>MSGAMAALTAEHFAALQSLLKASSKDVVRQLCQESFSSSALGLKKLLDVTCSSLSVTQEEAEELL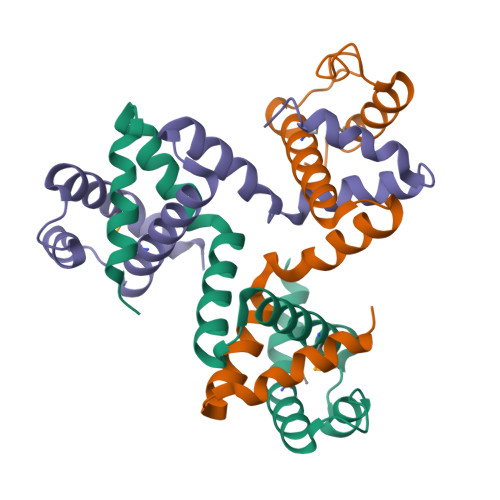QALHRMTRLVAFRDLSSAEAILALFPENFHQNLKNLLTKIMLEHVSTWRTEAQANQ[6x]>MGSSHHHHHHGTAENLYFQGERKYSTFYEQRATLFEELPVTSKDIIFLGNSITNGCEWAELFQNKNVKNRGISGDICMGVYDRLDPIVKGKPAKIFLLIGINDVSRGTSADKIISEISMIVRKIKQESPKTKLYLQSVLPVNDCYGMFNGHTSRWQVVKQINDLLEPLAVKEGVAYIDLYSHFVEKETGKMNPVYTNDGLHLLGKGYLLWRDIVKPYVDQK[8x]

Here, the crystal structure of a 9-O-SAE from Phocaeicola vulgatus (PvSAE) is reported. Structural characterization revealed PvSAE to be a dimer with an SGNH fold, named after the conserved sequence motif of this family, and a Ser–His–Asp catalytic triad. Biochemical assays also show that PvSAE deacetylates both mucin and the acetylated chromophore para-nitrophenyl acetate. Therefore, bacteria employ esterases to make acetylated sialic acid more accessible for cleavage by sialidases.

A crystal from the Apo I condition diffracted to a resolution of 1.44 Å and had P1211 symmetry, while a crystal from the Apo II condition diffracted to 2.06 Å resolution and had P61 symmetry. The unit cells of these crystals contained four and eight protomers for the Apo I and Apo II forms, respectively. These protomers were arranged as dimers in both crystal forms, recapitulating the dimeric form observed in solution. The PvSAE Apo I and Apo II structures displayed a near-complete overlap when aligned [root-mean-square deviation (r.m.s.d.) of 0.18 Å], with the secondary structures in the same conformation. The only major difference between these structures was a small region of the most N-terminal α-helix, which is discussed below. Mg2+ interacts with the carbonyl groups of Pro194 and Thr197, the side-chain hydroxyl group of Tyr146 and three waters. Docking into the ‘blocked’ site of the Apo I structure resulted in a ligand conformation with the 2-position projecting towards the N-terminal α-helix, suggesting that this active site could only accommodate monomeric substrates. A similar conformation to the blocked active site was observed in the Apo II structure.>[4x]MTMDTAQLKSQIQQYLVESGNYELISNELKARLLQEGWVDKVKDLTKSEMNINESTNFTQILSTVEPKALEMVSDSTRETVLKQIREFLEEIVDTQ;>GSTIDSISNGILNNLLTTLI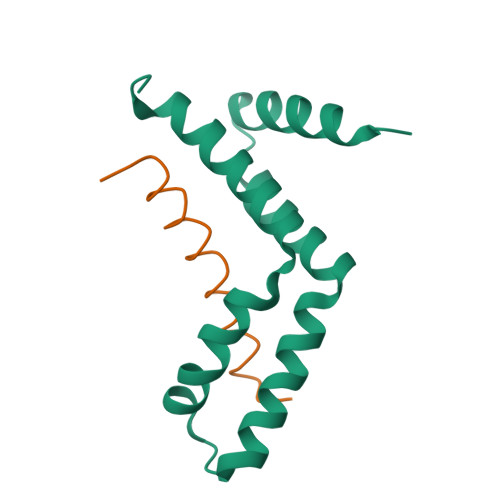QDIVARETT[4x]1,25-Dihydroxy-16-ene-20-cyclopropyl-vitamin D3 | 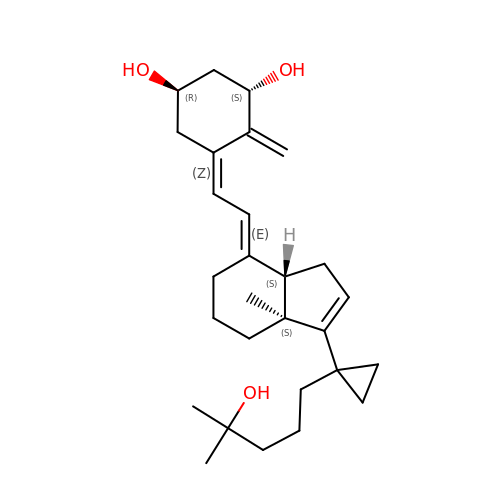C28 H42 O3 | WFPGMTGDYDCQLS-LMQQRSCXSA-N> AVFRSEADKKFKYSVKLSDYMTLQEAATAAVDSLLIDIDYNFIDGEAVDFGGKVLTIECKAKFIGDGVLNWNNLGSGSKVISPHMHTKTTPYTVYRFDDNGNWVTNPTTVLASVAQRLDKGYKPNVNDHDIWASLPDNVKNQVAGATLRVNSANNIIFTHPEATMGGYLFTLCNHILVESPRNFIAWESGITFENHHTTAWGTGNKVVGGEIKYGSGSAVLFIRNDG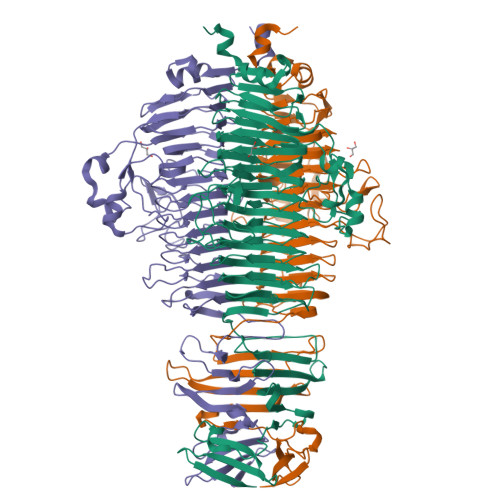GDDHDGGVRDLISYRVGESGVKTYQNEIGGRSARNYRLVFDNITTIQCYYDGIDVNADTGSPTERVDDYTLAEYPWFQLPTQHIIRNIITRDCMGIGAWWDGQKNIIDNVVTYEAHKEGMFDRGTNNDITNITVVCANKDLTNLNQIVCEGGSRLRGIMVHAYTTQGYAVYAPSSEVSNVSCAGSGTKKILCTYVADIQGGNINVQHGENAMTLSMRPAMGGTINPSLVLTADCQVASPGNEASIVKLSAIQDGARVGELQLNRLGFKHMSIPVAESQLPESALEFNSSIGFFFGTDDELRILAKKPDGTFVTYSL>[2x]MDSSQLHVAIVSSPGMGHLIPVLVLGNRLATHHNIKITILAITTTSSSAETEFLKKTTLTNEEKTIEIIPVPSVDISHLINSSTKIFTQLRLLVREALPKIHSTIASMTHRPDALIVDIFCTQILPIAEEFNISKYTYHPTTAWTLALAIYCQVFDKEIEGEYVELKEPLKIPGCKALRPDDVVDPLLDRSDQQYEEYVKLGKEYTDF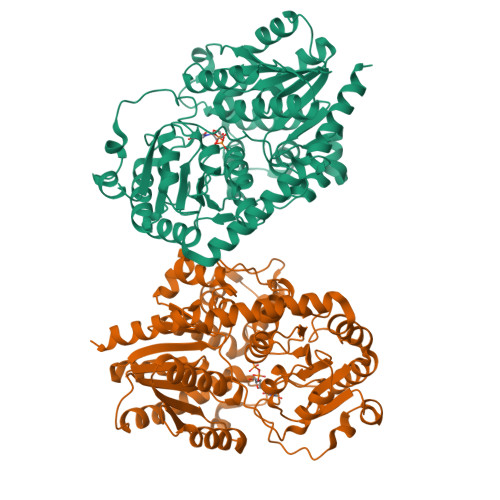DGILINTWEDLEPETINALRYNEKLRLLLKVPVFPIGPLRRKVETTLNDEVIQWLDKQNNESVLFVSFGSGGTLSTKQMTELAWGLELSQQKFVWVVRPPSDGDADSAYLNSAGKDTRDMSEYLPEGFLTRTKDMGLVVPMWANQVEILSHSSVGGFLTHCGWNSTVESLTNGVPMIAWPLHAEQKMNAAMLTEELGVAIRPAVLPTKKLVKREEIQGMVRILMQTKEGKRIKEKAKKLKKSAENALSDGGSSYNSICELVKDIRSREL>GSHMNGHIYAVGGYDGSPDGHTHLNSVEAYDPERDEWHLVAPMNTRRSGVGVAVLNGHIYAVGGFDGSPDGTDHLNSVERYDPERDEWRLVAPMNTRRSGVGVAVLNGHIYAVGGYDGSPDGHTHLNSVEAYDPERDEWHLVAPMNTRRSGVGVAVLNGHIYAVGGFDGSPDGTDHLNSVERYDPERDEWRLVAPMNTRRSGVGVAVLNGHIYAVGGYDGSPDGHTHLNSVEAYDPERDEWHLVAPMNTRRSGVGVAVLNGHIYAVGGFDG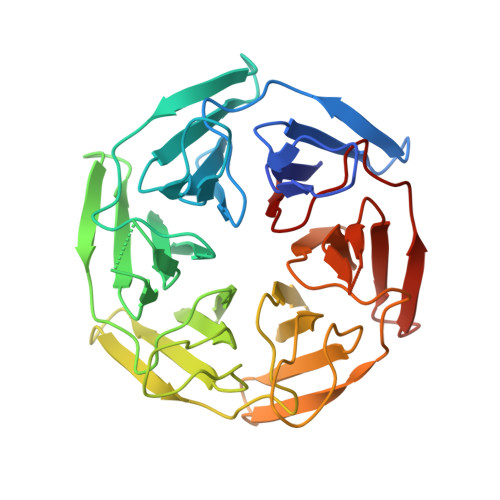SPDGTDHLNSVERYDPERDEWRLVAPMNTRRSGVGVAVL[4x]>[8x]MGSSHHHHHHAAPLPELLSNNGKHALMVDGAPYIILGSQTN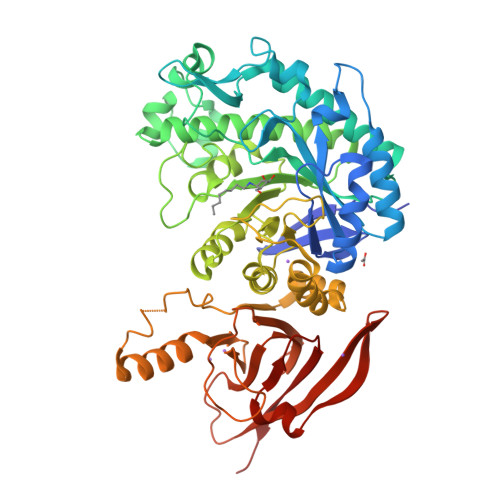NSSNYPDALKDVWPSMEKMGANTLSIPVAWEQIEPVEGQFDFSFVDVLLKEARQRKVRLVLLWFATWKNNAPHYAPAWVKLDNARFPRVVKEDGDTLNSLSPLGQNTLAADKKAFVELMKYLAKRDKDHTVIMVQVQNEVGTYGAVRDYSPMAQAVFNAAVPDDLIQKLQLKPGTWSQVFGRDADEFFHAYQIARYCDEVTVAGKAIKNLPMYVNVALRNPFNPGLPGQYSSGGGTDNVLHIWKAAAPNIDLIAPDIYFRDYKTVSKVLELYTRPDNALFVAEIGNDQPFARYLFPTLGKGGIGFSPFGMDDTDYTNYPLGAKVYNDETIEQFAQVYRLVNPMMREWARLSYQGQVWGVAEPLDSTTETQKIWNAEATPEEKEQHKKDRASALTQQLDLGLWDAEVTYGRPMFWVTPPEGNTPAAGGALIAQLDDNEYLVTAYKARVEFKPSQELAGKKFMIERVEEGRFEKGKWVMERVWNGDQTDWGLNFTDRPHLLRVKMASYSVQ>SNAPRTSTGTEPVHPPPAPSGINSPAPTPQPPPSGISAPPKTPASAPPPPVAKPAVFIPVNRTPEMQEERLKLPILAEEQAIMEAVAEHPIVIVCGETGSGKTTQVPQFLYEAGYSSEDSIIGVTEPRRVAAVAMSQRVAKEMNLSHRVVSYQIRYEGNVTEETRIKFMTDGVLLKEIQKDFLLLKYKVVIIDEAHERSVYTDILLGLLSRIVALRAKRHLPLKLLIMSATLRVEDFTQNQRLFTTPPPVIKVESRQFPVTVHFNKRTPLDDYSGECFRKVCKIHRMLPAGGILVFLTGQAEVHALCRRLRKAFPFRCSQPQEKEEDSAEGMRRFKKSRTRARKAQAMALPQINLDNYSVLPAGEGDEDREAEMDDEEEALGSDLDLDLGDSEANEGEQPDASLPLHVLPLYSLLAPEKQAQVFKPPPEGTRLCVVATNVAETSLTIPGIKYVVDCGKVKKRYYDRVTGVSSFRVTWVSQASADQRAGRAGRTEPGHCYRLYSSAVFGDFEQFPPPEITRRPVEDLILQMKALSIEKVINFPFPTPPSVEALVAAEELLVALGALQAPPKQERMKKLQMSQLSCPITALGRTMSTFPVAPRYAKMLALSQQHGCLPYTIAIV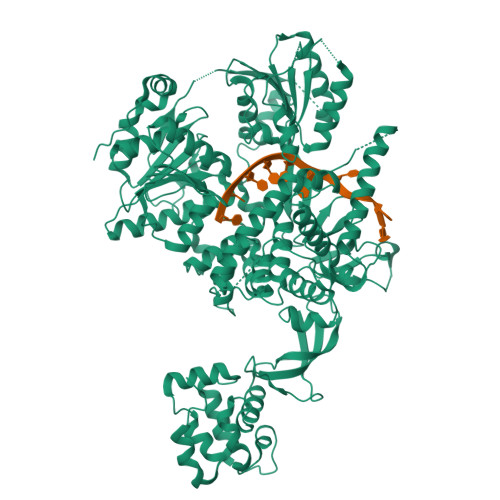AAMTVRELFEELDRPAASEKELAELKGRRARVAQMKRTWAGQGPSLKLGDLMVLLGAVGACEYAGCSPQFCQANGLRYKAMLEIRRLRGQLTTAVNAVCPEAGLFLDPKMQPPTESQVTYLRQIMAAGLGDHLARRVQSEDLLDPKWKNAYKTPLLDDPVFIHPSSVLFKELPEFVVYQEIVETTKMYMKGVSTVEIQWIPSLLPSYCQFDAPLEEPAPSYCPESGQVLCHRASVFYRVGWPLPAVQVDFPEGIDRYKYFAKFLLEGQVFRKLASFKSCLLSSPSTMLKTWARLQPRTETLLRALVAHKADSRDSLLAAWKKNPKYLLAEYCEWLPKAMHSDVEKNWPPTTDS[2x]> GSMLVLITYDVQTSSMGGTKRLRKVAKACQNYGQRVQNSVFECIVDSTQLTSLKLELTSLIDEEKDSLRIYRLGNNYK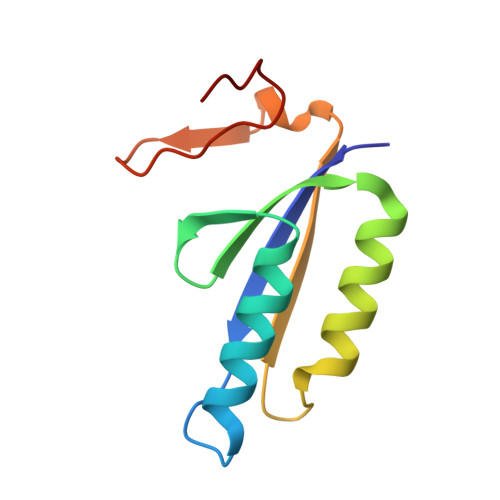TKVEHIGAKPSIDLEDPLIF>MFYEIRTYRLKNGAIPAYLKVVEDEGIEIQKSHLGELVGYFFSEIGPINEIVHIWAFSSLDD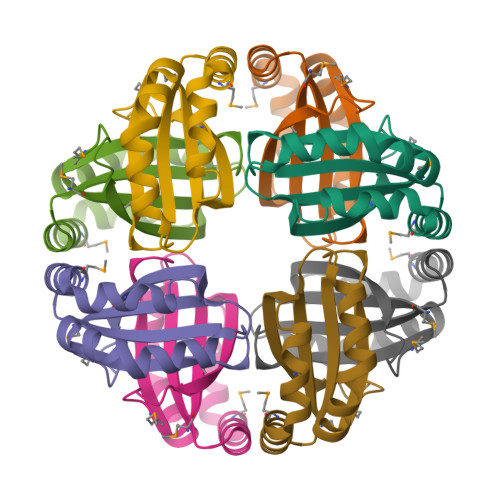RAERRARLMADPRWLSFLPKIRDLIEVAENKIMKPARFSPLMLEHHHHHH[8x]> MGFHFQQYIAMAGRAINP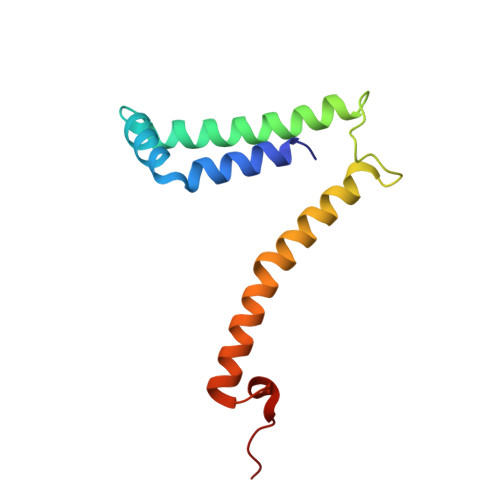VQWTRAWRRMEGKSATEVYRDALAWTNNQFAQISRASQYRAWWWQNPLGMGLVLYGTYKAWHMIYMVRKQKKTAQLVAAAYGQGGQWLNPVPR>[2x]DCMFGNGKGYRGKRVTTVTGT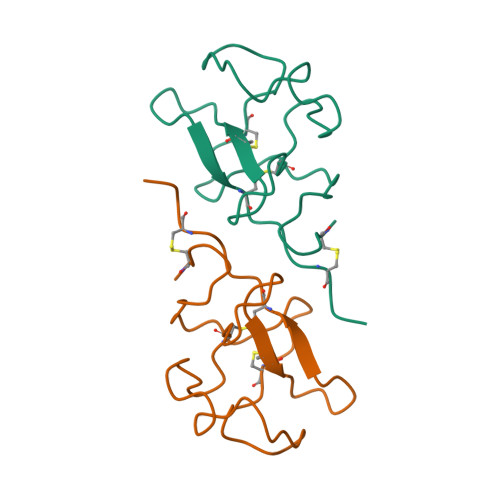PCQDWAAQEPHRHSIFTPETNPRAGLEKNYCRNPDGDVGGPWCYTTNPRKLYDYCDVPQCAAP>SNAMKIIILGAGQVGGTLAENLVGENNDITIVDKDGDRLRELQDKYDLRVVNGHASHPDVLHEAGAQDADMLVAVTNTDETNMAACQVAFTLFNTPNRIARIRSPQYLAQKEALFKSGAIPVDHLIAPEELVTSYIERLIQYPGALQVVSFAEEKVSLVAVKAYYGGPLVGNALSALREHMPHIDTRVAAIFRQGRPIRPQGTTIIEADDEVFFVAASNHIRSVMSELQRLEKPYRRIMIVGGGNIGASLAKRLEQTYSVKLIERNLQRAEKLSEELENTIVFCGDAADQELLTEENIDQVDVFIALTNEDETNIMSAMLAKRMGAKKVMVLIQRGAYVDLVQGGVIDVAISPQQATISALLTHVRRAD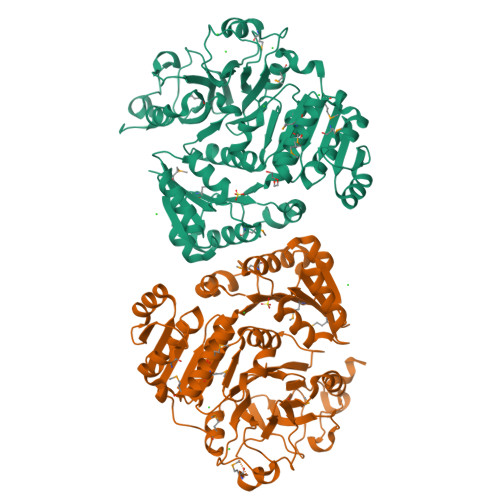IVNVSSLRRGAAEAIEAVAHGDESNSKVVGRAVGDIKLPPGTTIGAIVRGEEVLIAHDRTVIEQDDHVVMFLVDKKYVPDVEALFQPSPFFL[2x]Middle East respiratory syndrome coronavirus (MERS-CoV) has emerged as a highly fatal cause of severe acute respiratory infection. We developed an alternative vaccine regimen, based on full-length S DNA and a truncated S1 subunit glycoprotein, to elicit a broad repertoire of antibodies with diverse mechanisms of viral neutralization, and found that immunization with these constructs protected non-human primates (NHPs) from severe lung disease after intratracheal challenge with MERS-CoV. The England1 strain (GenBank ID: AFY13307) was chosen on the basis of the availability of its sequence and its proximity to a consensus among published sequences, particularly within the RBD. The final round of hybridoma screening generated 45 subclones, four of which (D12, F11, G2 and G4) were selected for additional characterization on the basis of their binding specificity and neutralization potency.

(d,e) Crystal structure of MERS England1 RBD and effect of critical RBD mutations on binding. RBD residues 506 and 509, identified by mutagenesis analysis, are highlighted in green. Critical RBD residues 532, 535 and 536, identified by structural definition and viral resistance evolution, reduce or eliminate D12 binding (shown in red). ELISA results show that this set of mutations eliminate F11 or D12 binding. Although it also targets the RBD, F11 neutralizes MERS-CoV by a different mechanism than D12. Site-directed mutagenesis and competition-binding studies indicate that F11 makes contact with the RBD on the opposing side of the binding site of D12, at and around residue 509. Binding studies also show that both D12 and F11 can bind to the RBD at the same time, suggesting the potential for additive neutralization effects.

>VECDFSPLLSGTPPQVYNFKRLVFTNCNYNLTKLLSLFSVNDFTCSQISPAAIASNCYSSLILDYFSYPLSMKSDLSVSSAGPISQFNYKQSFSNPTCLILATVPHNLTTITKPLKYSYINKCSRFLSDDRTEVPQLVNANQYSPCVSIVPSTVWEDGDYYRKQLSPLEGGGWLVASGSTVAMTEQLQMGFGITVQYGTDTNSVCPKL[2x]> MNHKVHHHHHHIEGRHMNATVETTQHDVEGTGAAGATAMLFPGMGPAAFSDVGRFMVTNRYTRELLAEADDTLGYSLVDRFRQAEGDYSEYAQIAFLVNCVALARWAEQTMDLTPRICAGASFGEKSVAAYSGALTFADAVRMTAGLARCMDEYFRTEHLGVVTHSFVRAPRERLDEILAELDERGEWHEISCHIDHDFFMLTLHERNSVWLEGRLRSVGAMPLYAMRPPMHAAAFGGLRDKAEEEVIAPLTFHDPTLPVVADQDGKVLTTGDEVRTMLLECFVRPLRWPDVISSLQDQGVTRVCVAGPDSLFGRVGTTTRAFEVIAATPRLALQPRARTTSR;> GS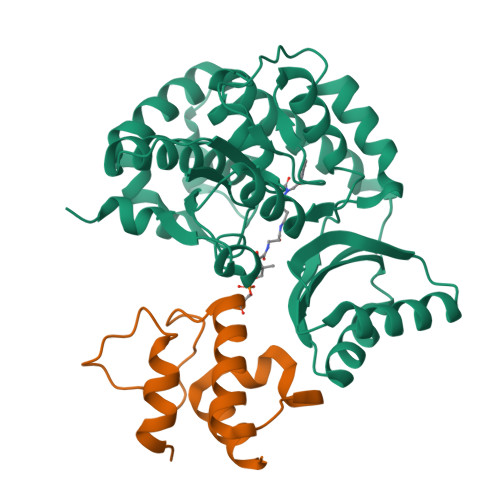HMWDAQFENLLRRYLPFLSADQPLEQDINLRDIGLDSLGTVELLSELENTYDVHFQDEALTKETFETPGVLWKTLSQMVEPRH1,4-oxazepane | C5 H11 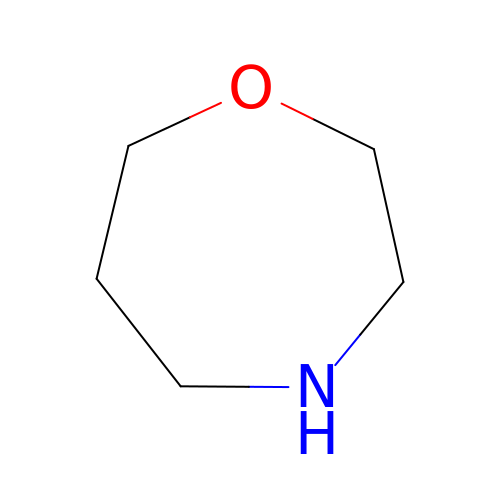N O | ZNGWEEUXTBNKFR-UHFFFAOYSA-N>ADKLFINALKKKFEESPEEKKTTFYTLGGWKQSERKTEFVNAGKEVAAKRGIPQYNPDIGTPLGQRVLMPYQVS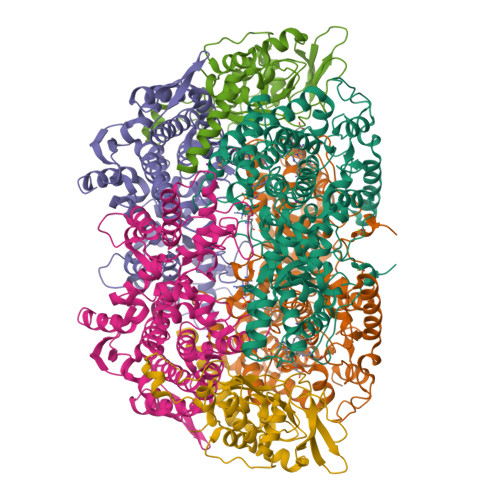TTDTYVEGDDLHFVNNAAMQQMWDDIRRTVIVGLNHAHAVIEKRLGKEVTPETITHYLETVNHAMPGAAVVQEHMVETHPALVADSYVKVFTGNDEIADEIDPAFVIDINKQFPEDQAETLKAEVGDGIWQVVRIPTIVSRTCDGATTSRWSAMQIGMSMISAYKQAAGEAATGDFAYAAKHAEVIHMGTYLPVRRARGENEPGGVPFGYLADICQSSRVNYEDPVRVSLDVVATGAMLYDQIWLGSYMSGGVGFTQYATAAYTDNILDDFTYFGKEYVEDKYGLCEAPNNMDTVLDVATEVTFYGLEQYEEYPALLEDQFGGSQRAAVVAAAAGCSTAFATGNAQTGLSGWYLSMYLHKEQHSRLGFYGYDLQDQCGASNVFSIRGDEGLPLELRGPNYPNYAMNVGHQGEYAGISQAPHAARGDAFVFNPLVKIAFADDNLVFDFTNVRGEFAKGALREFEPAGERALITPA[2x];>[2x]AKFEDKVDLYDDRGNLVEEQVPLEALSPLRNPAIKSIVQGIKRTVAVNLEGIENALKTAKVGGPACKIMGRELDLDIVGNAESIAAAAKEMIQVTEDDDTNVELLGGGKRALVQVPSARFDVAAEYSAAPLVTATAFVQAIINEFDVSMYDANMVKAAVLGRYPQSVEYMGANIATMLDIPQKLEGPGYALRNIMVNHVVAATLKNTLQAAALSTILEQTAMFEMGDAVGAFERMHLLGLAYQGMNADNLVFDLVKANGKEGTVGSVIADLVERALEDGVIKVEKELTDYKVYGTDDLAMWNAYAAAGLMAATMVNQGAARAAQGVSSTLLYYNDLIEFETGLPSVDFGKVEGTAVGFSFFSHSIYGGGGPGIFNGNHIVTRHSKGFAIPCVAAAMALDAGTQMFSPEATSGLIKEVFSQVDEFREPLKYVVEAAAEIKNEI;>AQYYPGTTKVAQNRRNFCNPEYELEKLREISDEDVVKILGHRAPGEEYPSVHPPLEEMDEPEDAIREMVEPIDGAKAGDRVRYIQFTDSMYFAPAQPYVRSRAYLCRYRGADAGTLSGRQIIETRERDLEKISKELLETEFFDPARSGVRGKSVHGHSLRLDEDGMMFDMLRRQIYNKDTGRVEMVKNQIGDELDEPVDLGEPLDEETLMEKTTIYRVDGEAYRDDVEAVEIMQRIHVLRSQGGFN[2x]>MIQGVIQKIAGPAVIAKGMLGARMYDICKVGEEGLVGEIIRLDGDTAFVQVYEDTSGLKVGEPVVSTGLPLAVELGPGMLNGIYDGIQRPLERIREKTGIYITRGVVVHALDREKKWAWTPMVKPGDEVRGGMVLGTVPEFGFTHKILVPPDVRGRVKEVKPAGEYTVEEPVVVLEDGTELKMYHTWPVRRARPVQRKLDPNTPFLTGMRILDVLFPVAMGGTAAIPGPFGSGKTVTQQSLAKWSNADVVVYVGCGERGNEMTDVLVEFPELTDPKTGGPLMHRTVLIANTSNMPVAAREASIYVGVTIAEYFRDQGFSVALMADSTSRWAEALREISSRLEEMPAEEGYPPYLAARLAAFYERAGKVITLGGEEGAVTIVGAVSPPGGDMSEPVTQSTLRIVGAFWRLDASLAFRRHFPAINWNGSYSLFTSALDPWYRENVAEDYPELRDAISELLQREAGLQEIVQLVGPDALQDAERLVIEVGRIIREDFLQQNAYHEVDAYCSMKKAYGIMKMILAFYKEAEAAIKRGVSIDEILQLPVLERIGRARYVSEEEFPAYFEEAMKEIQGAFKALA[3x];>[3x]MDLLKKEYTGITYISGPLLFVENAKDLAYGAIVDIKDGTGRVRGGQVIEVSEEYAVIQVFEETTGLDLATTSVSLVEDVARLGVSKEMLGRRFNGIGKPIDGLPPITPEKRLPITGLPLNPVARRKPEQFIQTGISTIDVMNTLVRGQKLPIFSGSGLPANEIAAQIARQATVRPDLSGEGEKEEPFAVVFAAMGITQRELSYFIQEFERTGALSRSVLFLNKADDPTIERILTPRMALTVAEYLAFEHDYHVLVILTDMTNYCEALREIGAAREEIPGRRGYPGYMYTDLATIYERAGVVEGKKGSVTQIPILSMPDDDRTHPIPDLTGYITEGQIQLSRELHRKGIYPPIDPLPSLSRLMNNGVGKGKTREDHKQVSDQLYSAYANGVDIRKLVAIIGEDALTENDRRYLQFADAFERFFINQGQQNRSIEESLQIAWALLSMLPQGELKRISKDHIGKYYGQKLEEIWGAPQALD;> MSQVSPTRMNLLQRRGQLRLAQKGVDLLKKKRDALVAEFFGLVREAMEARKALDQAAKEAYAALLLAQAFDGPEVVAGAALGVPPLEGVEAEVENVWGSKVPRLKATFPDGALLSPVGTPAYTLEASRAFRRYAEALIRVANTETRLKKIGEEIKKTTRRVNALEQVVIPGIRAQIRFIQQVLEQREREDTFRLKRIKGKIEAREAEEEGGRPNPQVEIGAGL;> MAVIADPETAQGFRLAGLEGYGASSAEEAQSLLETLVERGGYALVAVDEALLPDPERAVERLMRGRDLPVLLPIAGLKEAFQGHDVEGYMRELVRKTIGFDIKL

The V/A-ATPase from a thermophilic bacterium, Thermus thermophilus (Tth V/A-ATPase) is a rotary ATPase that has been well characterized using both structure and single molecular observation studies. The Tth V1 moiety is composed of four subunits with a stoichiometry of A3B3D1F1 and it is responsible for ATP synthesis or hydrolysis. The Tth Vo moiety, responsible for proton translocation across the membrane, contains a central rotor complex (d1c12) and stator apparatus made up of the a subunit and two EG peripheral stalks (a1E2G2). In the holo Tth V/A-ATPase, pmf drives rotation of the d1c12 rotor complex relative to the surrounding stator, resulting in rotation of the entire central rotor complex (D1F1d1c12) and inducing sequential conformation changes in the A3B3 catalytic hexamer to produce three ATP molecules from ADP and inorganic phosphates per one rotation.

We reconstructed the 3D structure of the holo complex rotational state 1 using 71,196 polished single particle images. The final structure of the state one has an overall resolution of 3.6 Å. After subtracting the EM density of the membrane embedded domain from the density of the whole complex, we obtained a focused density map of A3B3D1F1d1 with two EG peripheral stalks and the soluble arm domain of the a subunit (asol) at 3.5 Å resolution. This map allowed us to build an atomic model of A3B3D1F1 (V1). The secondary ADP in the semi-closed site shows a lower occupancy due to low affinity of the semi-closed site for the nucleotide and partial flexibility of the complex. Upon dissociation from Vo, the isolated V1 moiety displays only ATP hydrolysis activity accompanied by rotation of the DF shaft.>[2x]MKANNPQHSLTKDEIKQYIKEYVQAAKNSIAA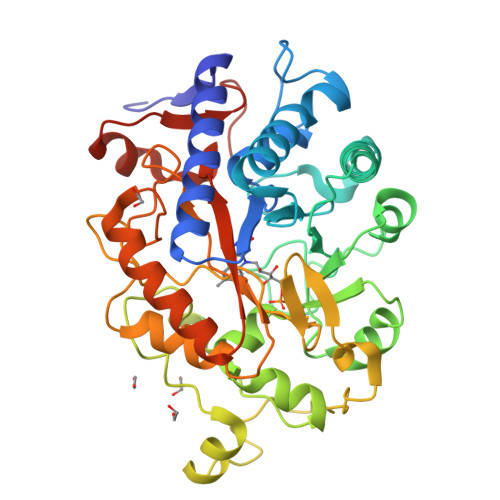GADGVEIHSANGYLLNQFLDPHSNTRTDEYGGSIENRARFTLEVVDALVEAIGHEKVGLRLSPYGVFNSMSGGAETGIVAQYAYVAGELEKRAKAGKRLAFVHLVEPRVTNPFLTEGEGEYEGGSNDFVYSIWKGPVIRAGNFALHPEVVREEVKDKRTLIGYGRFFISNPDLVDRLEKGLPLNKYDRDTFYQMSAHGYIDYPTYEEALKLGWGTSSFVKDFKPQALGDTNLFKPIKIGNNELLHRAVIPPLTRMRALHPGNIPNRDWAVEYYTQRAQRPGTMIITEGAFISPQAGGYDNAPGVWSEEQMVEWTKIFNAIHEKKSFVWVQLWVLGWAAFPDNLARDGLRYDSASDNVFMDAEQEAKAK>AQVINTFDGVADYLQTYHKLPDNYITKSEAQALGWVASKGNLADVAPGKSIGGDIFSNREGKLPGKSGRTWREA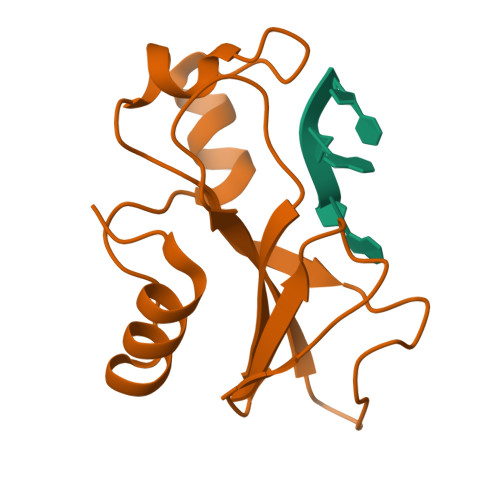DINYTSGFRNSDRILYSSDWLIYKTTDHYQTFTKIR[2x]>HHHHHHSSGLVPRGSMDIRALYDEKLTTPEEAVSSIASGSHLSMGMFAAEPPALLKALADRATRGDIGDLRVYYFETAKIAGDTILRYELNNRIKPYSMFVTAVERALIRRGIEDGGRKVVNYVPSNFHQAPRLLAEEIGIDTFMHTVSPMDCHGYFSLGVGNDYSSRIARSARRFIVEVNRYMPRVQGEAAAIHISEVDAIVENHVPLIEMPVRSAIPEYTSISHIIADLVPDGACLQMGVGALPNLVCGVLKDRNDLGIHTEVLNPGLVDLIRRGVVTNQRKTLDRGRSVFTFAMGQQEMYEYLNDHPAIFSRPVDYVNDPHIIAQNDNVVSINATLQIDLTGACNSEHMLGHQYSASGGQLDFVRGAYASKGGRSIIATPSTAAKGTVSRIIPRIDGPVTTPRIDTHYIVTEFGAVNLKGLSSTERALRI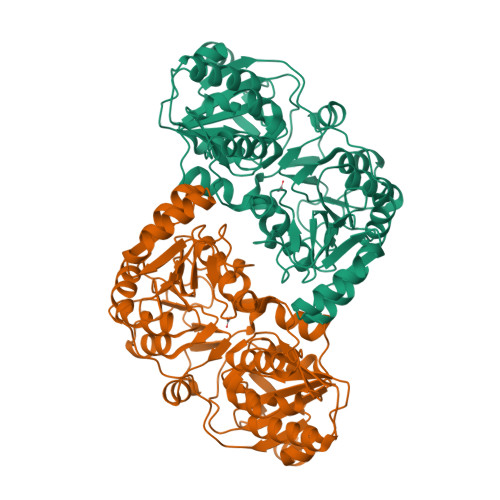IELAHPDFRDELTQAAKKMHLI[2x]>AMGAAELRFCNQTIKELMSKKHYNYNFPFLAPVDTVALNIPNYNEIVKQPMDLGTIQSKLANNEYENADDFEKDVRLVFKNCYLFNPEGTDVNMMGHRLEAVFDKKWAN[2x]

BET proteins are chromatin-associated factors that regulate transcription and chromatin remodelling. BET proteins bind chromatin through their two BDs (BD1 and BD2), which specifically recognize histones acetylated on lysine residues. The BDs from C. albicans Bdf1 (CaBdf1) share 31–46% sequence identity with human BET BDs and 58–66% identity with those from ScBdf1 and hence are likely to bind multi-acetylated H3 and H4 tails. In conclusion, Bdf1 BDs are required for the viability and virulence of C. albicans and can be selectively targeted by small-molecule inhibitors without compromising human BET BD function.

Similarly, we identified an imidazopyridine compound 2, which inhibits CaBdf1 BD2 with high selectivity: HTRF and ITC assays yielded IC50 and Kd values of 1.1 and 2.1 μM, respectively, whereas human Brd4 BD2 and CaBdf1 BD1 were only weakly inhibited (IC50≥40 μM). Moreover, no significant inhibition of any human BDs was observed for compound 2 by BROMOscan profiling and by an ITC assay on the two most sensitive BDs identified by this screen (SMARCA2 and SMARCA4); while only mild cytotoxicity was observed towards mammalian cells (EC50 ∼60 μM). The crystal structure of CaBdf1 BD2 bound to 2 reveals that the compound forms a hydrogen bond via its amino group with the conserved Asn468 residue, as well as a cation–pi interaction involving the phenolic ring and the partial positive charge on Asn468. However, unlike most BET inhibitors, a water-mediated hydrogen bond with Tyr425 is not observed for 2 (presumably because the ligand dislodges water molecule 1, consistent with the dislodgement of this water by a glycerol molecule in the unbound BD structure; Supplementary Fig. 3d). Instead, the compound's imidazolyl and hydroxyl groups form water-mediated hydrogen bonds with backbone atoms of the Phe-Pro-Phe (FPF) shelf (Pro410) and helix B (Val460). Replacement of the hydroxyl group in 2 by a hydrogen (2a) or fluorine (2b) atom severely reduces inhibitory activity, underscoring the importance of this group for high-affinity binding. The methylpyridinyl and phenolic groups are sandwiched between the FPF shelf and gatekeeper residue Val474 on one side, and residues Val415 and Leu420 on the other, while the tolyl group additionally contacts residues Ile422 and Phe467. A structural alignment with Brd4 BD2 shows that larger Brd4 side chains at four of these contact positions, including signature positions 1,3 and 5 (Trp374, Leu387 and His437) and residue Tyr432, reduces the volume available for compound 2, explaining the inability of 2 to inhibit the human BD. In contrast, the poor affinity for CaBdf1 BD1 is due to smaller side chains at signature positions 1 and 3 (Val232 and Val245), resulting in poor complementarity between the binding pocket and ligand. The selectivity of 1 and 2 for CaBdf1 results from steric incompatibility with bulkier side chains in the human BET BD-binding pockets, particularly at signature positions 1 and 3.> MFQTFISRHNSNFFSDKLVLTSVTPASSAPVLQTPKATSSTLYFDSLTVNAGNGGFLHCIQMDTSVNAANQVVSVGADIAFDADPKFFACLVRFESSSVPTTL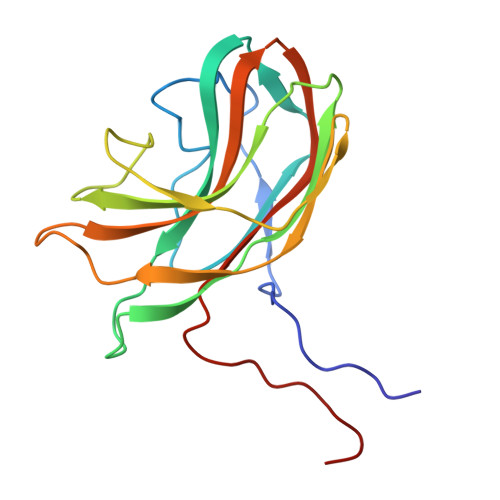PTAYDVYPLNGRHDGGYYTVKDCVTIDVLPRTPGNNVYVGFMVWSNFTATKCRGLVSLNQVIKEIICLQPLK Here, we report a general and rapid method for discovering α-helically constrained (Helicon) polypeptides that cooperatively induce the interaction between two target proteins without relying on previously known binders or an intrinsic affinity between the proteins. We show that Helicons are capable of binding every major class of E3 ubiquitin ligases, which are of great biological and therapeutic interest but remain largely intractable to targeting by small molecules. In addition to possessing increased stability and membrane permeability, Helicons are capable of binding large, flat protein surfaces that are inaccessible to targeting by small molecules, and Helicons have been developed to target a range of PPI targets in cells and in vivo. Characterizing Helicon-E3 co-structures and mechanisms of action, we identified new binding sites for α-helices on the E3 surfaces, as well as potential probes of the disease-linked E3, WWP123,24, highlighting the generality of our approach against this therapeutically important target class.

We performed screens to find Helicons that bind to CRLs consisting of Cullin proteins paired with their canonical adapter proteins. We identified Helicon hits forming VHL-ELOBC-specific clusters and CUL5-specific clusters. Among the CUL5-binding Helicons, H314 from C76 bound with a KD of 530 nM as assessed by SPR. H314 also disrupts the SOCS2-ELOBC:CUL5 interaction in a competition SPR (ABA) binding assay, potentially by competing for the adapter-binding site of CUL5. We further characterized by x-ray crystallography Helicons derived from these screens. We solved the structure of H314 with the CUL5 N-terminal domain (CUL5NTD) at ~2.8 Å resolution, H313 in complex with VHL-ELOBC at ~3.5 Å resolution, and CUL4B-specific H316 from C77 in complex with the N-terminal domain of CUL4B (CUL4BNTD) at ~2.9 Å resolution. H314 binds at the very N-terminus of CUL5, the binding site of the adapter complex SOCS2-ELOBC, consistent with its disruption of the CUL5 interaction with ELOBC in SPR assays. For instance, both the H314-binding site on CUL5 and the H313-binding site on VHL face the Ub-E2 binding sites of the cognate Cullin CTDs, providing a potentially ideal configuration for TPD applications, where both the E3 binding site and the ‘linkerology’ of heterobifunctional molecules is critically important to optimize ternary complex formation and the geometry of the E2- and E3-catalyzed reactions.

> SMATSNLLKNKGSLQFEDKWDFMRPIVLKLLRQESVTKQQWFDLFSDVHAVCLWDDKGPAKIHQALKEDILEFIKQAQARVLSHQDDTALLKAYIVEWRKFFTQCDILPKPFCQLEITLMGKQGSNKKSNVEDSIVRKLMLDTWNESIFSNIKNRLQDSAMKLVHAERLGEAFDSQLVIGVRESYVNLCSNPEDKLQIYRDNFEKAYLDSTERFYRTQAPSYLQQNGVQNYMKYADAKLKEEEKRALRYLETRRECNSVEALMECCVNALVTSFKETILAECQGMIKRNETEKLHLMFSLMDKVPNGIEPMLKDLEEHIISAGLADMVAAAETITTDSEKYREQLDTLFNRFSKLVKEAFQDDPRFLTARDKAYKAVVNDATIFKLE;> XDPAWYDCADAAWICTFX> LPL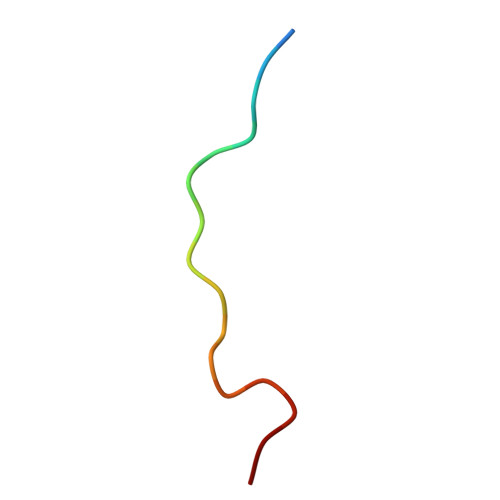YTSPSLPNITLGLP> MALSEIETRHSEIIKLENSIRELHDMFMDMAMLVESQGE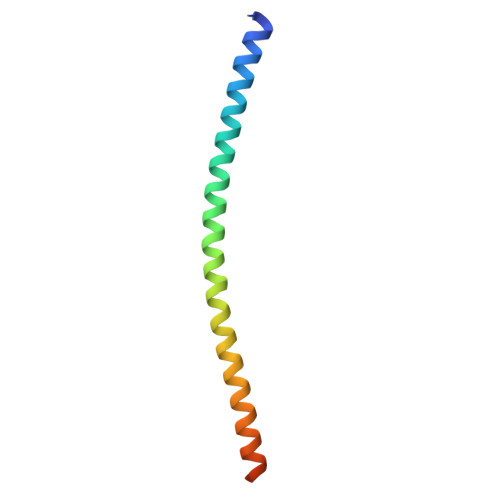MIDRIEYNVEHAVDYVERAVSDTKKAVKYQSKARRKKIM>MEFGFWSALYIFVLTCFLGYELITRVPVILHTPLMSGSNFIHGVVVVGAMVVLGHAETGLEKLIGFLGVILGAANAAGGYAVTVRMLEMFERKP[2x];>MDLIQAAYFVVAILFIVGLKRMAHPTTAKSGIVWAGWGMVLAVLATFFWPGMGNFALILLALLLGSVVAWWAAVRVAMTDMPQMVAIYNGMGGGAAATIAAVELLKGAFENTGLMALAILGGLIGSVAFTGSLIAFAKLQGIMKSRPILFPGQKAVNALVLALTVVIGLSLLWNDATASIVLFFLLALLFGVLMTLPIGGGDMPVAISFYNAFTGMAVGFEGFAVGNPALMVAGTLVGAAGTLLTVLMARAMNRSVWISVLVGGHH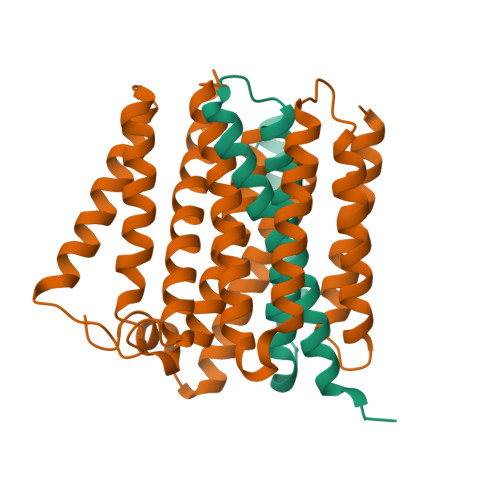HHHH[2x]>[2x]MEDVEIKPRGYQLRLVDHLTKSNGIVYLPTGSGKTFVAILVLKRFSQDFDKPIESGGKRALFMCNTVELARQQAMAVRRCTNFKVGFYVGEQGVDDWTRGMWSDEIKKNQVLVGTAQVFLDMVTQTYVAL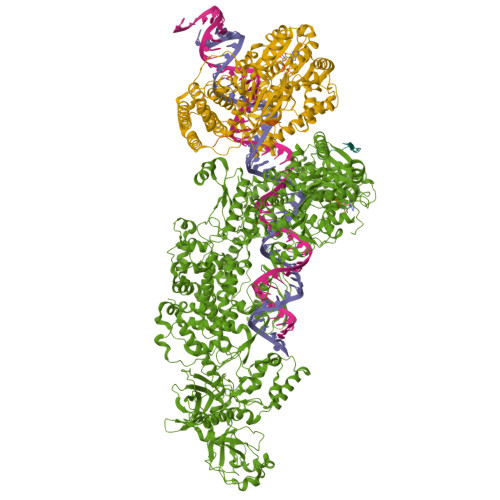SSLSVVIIDECHHGTGHHPFREFMRLFTIANQTKLPRVVGLTGVLIKGNEITNVATKLKELEITYRGNIITVSDTKEMENVMLYATKPTEVMVSFPHQEQVLTVTRLISAEIEKFYVSLDLMNIGVQPIRRSKSLQCLRDPSKKSFVKQLFNDFLYQMKEYGIYAASIAIISLIVEFDIKRRQAETLSVKLMHRTALTLCEKIRHLLVQKLQDMTYDDDDDNVNTEEVIMNFSTPKVQRFLMSLKVSFADKDPKDICCLVFVERRYTCKCIYGLLLNYIQSTPELRNVLTPQFMVGRNNISPDFESVLERKWQKSAIQQFRDGNANLMICSSVLEEGIDVQACNHVFILDPVKTFNMYVQSKGRARTTEAKFVLFTADKEREKTIQQIYQYRKAHNDIAEYLKDRVLEKTEPELYEIKGHFQDDIDPFTNENGAVLLPNNALAILHRYCQTIPTDAFGFVIPWFHVLQEDERDRIFGVSAKGKHVISINMPVNCMLRDTIYSDPMDNVKTAKISAAFKACKVLYSLGELNERFVPKTLKERVASIADVHFEHWNKYGDSVTATVNKADKSKDRTYKTECPLEFYDALPRVGEICYAYEIFLEPQFESCEYTEHMYLNLQTPRNYAILLRNKLPRLAEMPLFSNQGKLHVRVANAPLEVIIQNSEQLELLHQFHGMVFRDILKIWHPFFVLDRRSKENSYLVVPLILGAGEQKCFDWELMTNFRRLPQSHGSNVQQREQQPAPRPEDFEGKIVTQWYANYDKPMLVTKVHRELTPLSYMEKNQQDKTYYEFTMSKYGNRIGDVVHKDKFMIEVRDLTEQLTFYVHNRGKFNAKSKAKMKVILIPELCFNFNFPGDLWLKLIFLPSILNRMYFLLHAEALRKRFNTYLNLHLLPFNGTDYMPRPLEIDYSLKRNVDPLGNVIPTEDIEEPKSLLEPMPTKSIEASVANLEITEFENPWQKYMEPVDLSRNLLSTYPVELDYYYHFSVGNVCEMNEMDFEDKEYWAKNQFHMPTGNIYGNRTPAKTNANVPALMPSKPTVRGKVKPLLILQKTVSKEHITPAEQGEFLAAITASSAADVFDMERLEILGNSFLKLSATLYLASKYSDWNEGTLTEVKSKLVSNRNLLFCLIDADIPKTLNTIQFTPRYTWLPPGISLPHNVLALWRENPEFAKIIGPHNLRDLALGDEESLVKGNCSDINYNRFVEGCRANGQSFYAGADFSSEVNFCVGLVTIPNKVIADTLEALLGVIVKNYGLQHAFKMLEYFKICRADIDKPLTQLLNLELGGKKMRANVNTTEIDGFLINHYYLEKNLGYTFKDRRYLLQALTHPSYPTNRITGSYQELEFIGNAILDFLISAYIFENNTKMNPGALTDLRSALVNNTTLACICVRHRLHFFILAENAKLSEIISKFVNFQESQGHRVTNYVRILLEEADVQPTPLDLDDELDMTELPHANKCISQEAEKGVPPKGEFNMSTNVDVPKALGDVLEALIAAVYLDCRDLQRTWEVIFNLFEPELQEFTRKVPINHIRQLVEHKHAKPVFSSPIVEGETVMVSCQFTCMEKTIKVYGFGSNKDQAKLSAAKHALQQLSKCDA;>[2x]MDQENFHGSSLPQQLQNLHIQPQQASPNPVQTGFAPRRHYNNLVGLGNGNAVSGSPVKGAPLGQRHVKLKKEKISAQVAQLSQPGQLQLSDVGDPALAGGSGLQGGVGLMGVILPSDEALKFVSETDANGLAMKTPVSILQELLSRRGITPGYELVQIEGAIHEPTFRFRVSFKDKDTPFTAMGAGRSKKEAKHAAARALIDKLIGAQLPESPSSSAGPSVTGLTVAGSGGDGNANATGGGDASDKTVGNPIGWLQEMCMQRRWPPPSYETETEVGLPHERLFTIACSILNYREMGKGKSKKIAKRLAAHRMWMRLQETPIDSGKISDSICGELEGEVSIIQDIDRYEQVSKDFEFIKI>[2x]MSGPSGTAAASSSLVSESVVSLAAGT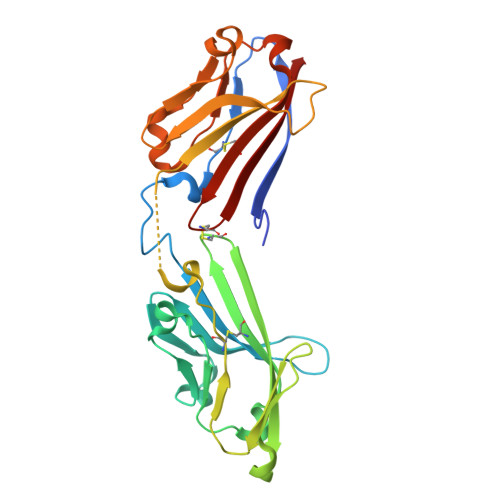QAVLRCQSPRMVWTQDRLHDRQRVVHWDLSGGPGSQRRRLVDMYSAGEQRVYEPRDRDRLLLSPSAFHDGNFSLLIRAVDRGDEGVYTCNLHHHYCHLDESLAVRLEVTEDPLLSRAYWDGEKEVLVVAHGAPALMTCINRAHVWTDRHLEEAQQVVHWDRQLPGVSHDRADRLLDLYASGERRAYGPPFLRDRVSVNTNAFARGDFSLRIDELERADEGIYSCHLHHHYCGLHERRVFHLQVT>MTLADSGTDFSTSNLVAVEPGAIREDTPPGSVIQYSDYELDTSSPYAGGAAWIEGEYVPASEARISIFDTGFGHSDLTYTVAHVWHGNIFRLADHIERLLDGARKLRLASPYDETEIAEIAKRCVGLSQLREAYVNITLTRGYGKRKGEKDLSKLTSQIYVYAIPYLWAFPPYEQIFGTSAVVPRHVQRAGRNTIDPTIKNYQWGDLTAASFEAKDRGARTGILLDADGCVAEGPGFNVVVVKDGALASPSRNALPGITRKTVFEIAHARGISAELRDVTSRELYDADELMAVTTAGGVTPITSLDGAAVGDGEPGPITVAIRDRFWALMDEPSDLI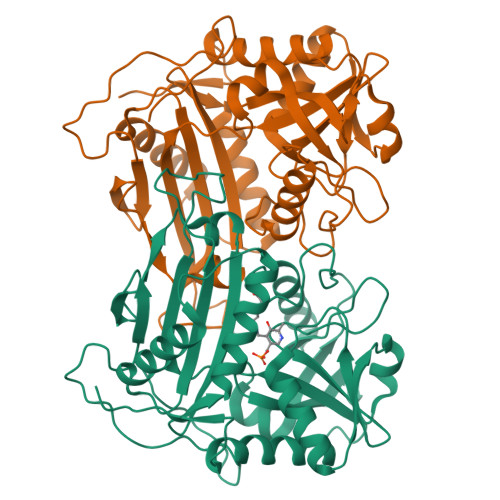DTIRYDVDRLE[4x]>[4x]GPLGSRHVACLARSERGLGFSIAGGKGSTPY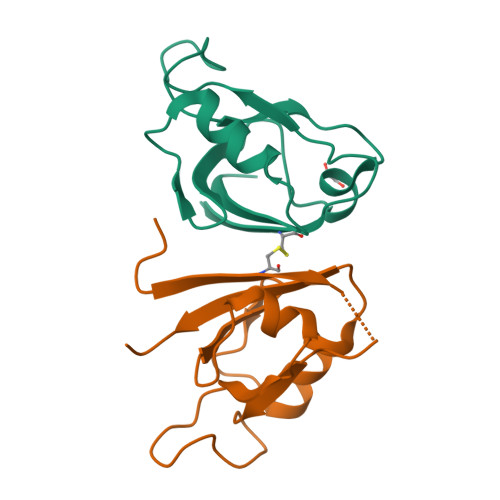RAGDAGIFVSRIAEGGAAHRAGTLQVGDRVLSINGVDVTEARHDHAVSLLTAASPTIALLLEREA> MALLAEHLLKPLPADKQIETGPFLEAVSHLPPFFDCLGSPVFTPIKADISGNITKIKAVYDTNPAKFRTLQNILEVEKEMYGAEWPKVGATLALMWLKRGLRFIQVFLQSICDGERDENHPNLIRVNATKAYEMALKKYHGWIVQKIFQAALYAAPYKSDFLKALSKGQNVTEEECLEKIRLFLVNYTATIDVIYEMYTQMNAELNYK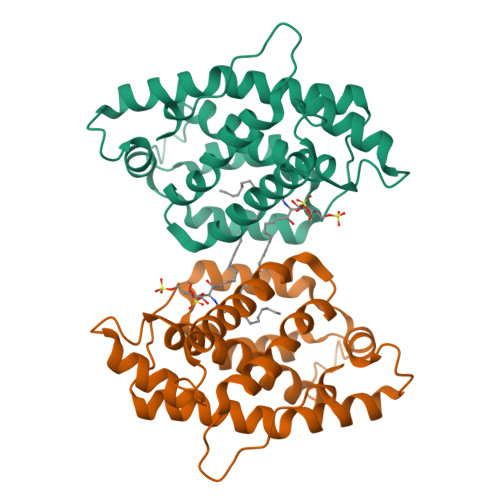V>GPHMFEARLVQGSILKKVLEALKDLINEACWDISSSGVNLQSMDSSHVSLVQLTLRSEGFDTYRCDRNLAMGVNLTSMSKILKCAGNEDIITLRAEDNADTLALVFEAPNQEKVSDYEMKLMDLDVEQLGIPEQEYSCVVKMPSGEFARICRDLSHIGDAVVISCAKDGVKFSASGELGNGNIKLSQTSNVDKEEEAVTIEMNEPVQLTFALRYLNFFTKATPLSSTVTLSMSADVPLVVEYKIADMGHLKYYLAPKIEDEEGS[3x];>RKAENKYAGGN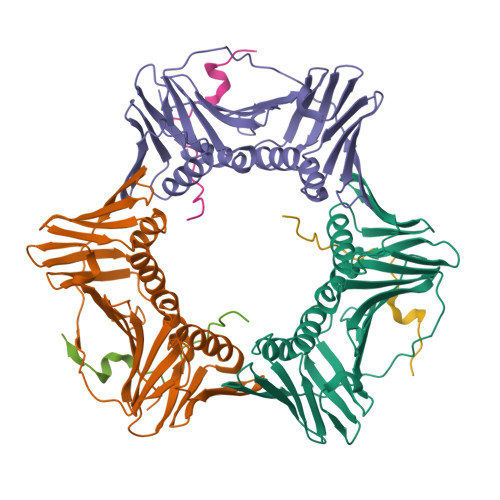PVCVRPTPKWQKGIGEFFRLS[3x]>SNAMKIKKESLEMRQMRKKVVLIGTGLIGGSLALAIKKDHDVTITGYDIFQEQVERAKELHVVDEIAVDLQHACEEAHLIVFASPVEETKKLLHKLASFHLREDVIVTDVGSTKGSIMNEAEALFSKEISFIGGHPMAGSHKTGVESAKAHLFENAFYILTPMHH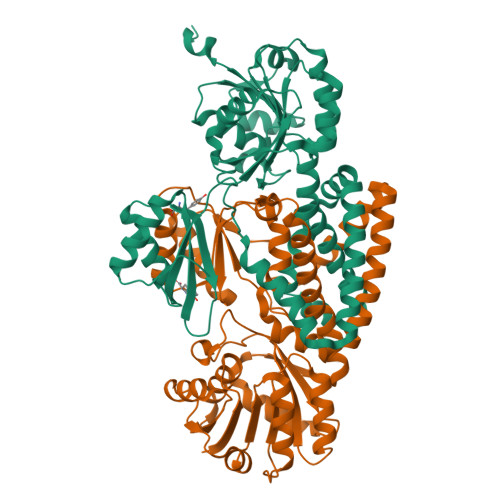VPNEHVEELKDWLKGTGSHFLVLNTEEHDYVTGIVSHFPHLIAAGLVKQVEKHAGDNPLIHQLAAGGFKDITRIASSSPKMWSDIVKQNREHLMVLLKEWISEMEDLYDTVSSGDAGEIQNYFADAKEYRDSLPVRKRGAIPAYHDLYVDVLDKVGALAHVTSILAREEISITNLQILEAREGLLGVLRISFQREEDRMKAKLALGEEKYQTYETI[4x]APOBEC3 proteins (A3s) are enzymes that catalyze the deamination of cytidine to uridine in single-stranded DNA (ssDNA) substrates, thus playing a key role in innate antiviral immunity. However, the APOBEC3 family has also been linked to many mutational signatures in cancer cells, which has led to an intense interest to develop inhibitors of A3’s catalytic activity as therapeutics as well as tools to study A3’s biochemistry, structure, and cellular function. Recent studies have shown that ssDNA containing 2′-deoxy-zebularine (dZ-ssDNA) is an inhibitor of A3s such as A3A, A3B, and A3G, although the atomic determinants of this activity have remained unknown. Analogous to the CDAs, A3s also depend on a Zn2+ located at the center of the substrate binding pocket, and the deamination reaction proceeds via a tetrahedral intermediate.

Here, we present the 1.5 Å resolution co-crystal structure of a soluble variant of human A3G catalytic domain (A3G-CTD2) bound to a 9-nucleotide ssDNA inhibitor containing 2′-deoxy-zebularine at the target position, 5′-AATCCdZAAA (dZ-ssDNA). The structure was solved in the space group P21 and contains a single A3G-CTD2:dZ-ssDNA complex in the asymmetric unit, similar to the previous co-crystal structure of A3G-CTD2* with ssDNA substrate. Given that our structure features the active A3G enzyme, we observed that 2′-deoxy-zebularine was converted to a tetrahedral hydration product; 4-(R)-hydroxy-3,4-dihydro-2′-deoxy-zebularine (dZ-H2O). In this hydration product, the N3 nitrogen of the zebularine nucleobase has become protonated, and a hydroxyl group added to the top face of the C4 carbon. Direct coordination of the C4-OH to the Zn2+ ion is evident by the short Zn2+-O distance (2.01 Å) and continuous electron density around the Zn coordination sites. The side chain carboxylate of E259 makes two hydrogen bonds, to both the N3-H and Zn-coordinated C4-O. The oxygen of the C4-OH, is directly coordinated to the 4th Zn-coordination site, replacing the Zn-bound water molecule seen in the previous structure of inactive A3G. This provides direct structural evidence of the second step of the deamination mechanism, whereby the Zn-coordinated hydroxide has attacked the top face of the 2′-deoxy-zebularine C4 carbon, forming a tetrahedral transition state intermediate. The pyrimidine ring of the hydrated 2′-deoxy zebularine (dZ-H2O) tilts upward ~8o when compared to the target cytosine (C0) in our previous A3G-CTD2*:ssDNA structure. In addition, the Zn2+ ion is pulled down ~0.8 Å from the inactive A3G-CTD2*:ssDNA structure. The A3G-CTD2:dZ-ssDNA structure provides clear structural evidence for the activation of dZ to a transition state analog and explains the stronger binding affinity and inhibitory activity seen for catalytically active A3 enzymes.

> GPLGSEILRHSMDPATFTFNFNNEPWVRGRHETYLCYEVERMHNDTWVKLAQRRGFLANQAKHKHGFLEGRHAELCFLDVIPFWKLDLDQDYRVTCFTSWSPCFSCAQEMAKFISKNKHVSLCIKTARIYDDKGRAAEGLRTLAEAGAKISIMTYSEFKHCWDTFVDHQGAPFQPWDGLDEHSQDLSGRLRAILQNQEN> GKVA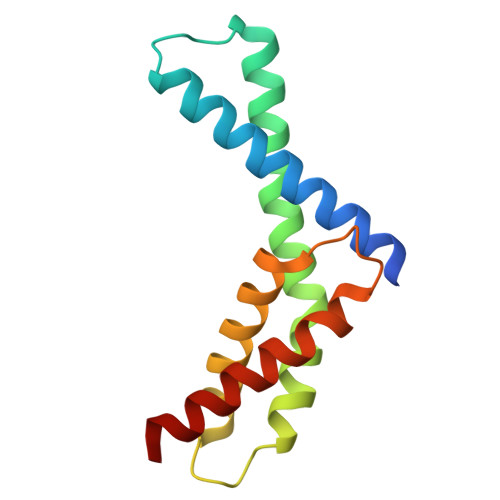LLNAEEEVELAKRIEAGLYATQLMTELSERGEKLPAAQRRDMMWICRDGDRAKNHLLEANLRLVVSLAKRYTGRGMAFLDLIQEGNLGLIRAVEKFDYTKGYKFSTYATWWIRQAITRAMADQAR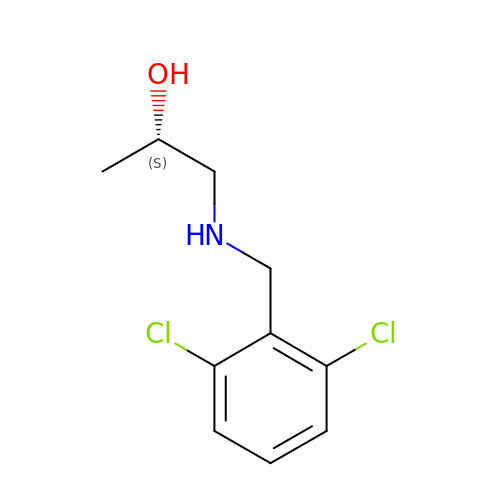(2S)-1-{[(2,6-dichlorophenyl)methyl]amino}propan-2-ol | C10 H13 Cl2 N O | BNJMFYUVZZATLR-ZETCQYMHSA-N>[2x]GEIRPTIGQQMETGDQRFGDLVFRQLAPNVWQHTSYLDMPGFGAVASNGLIVRDGGRVLVVDTAWTDDQTAQILNWIKQEINLPVALAVVTHAHQDKMGGMDALHAAGIATYANALSNQL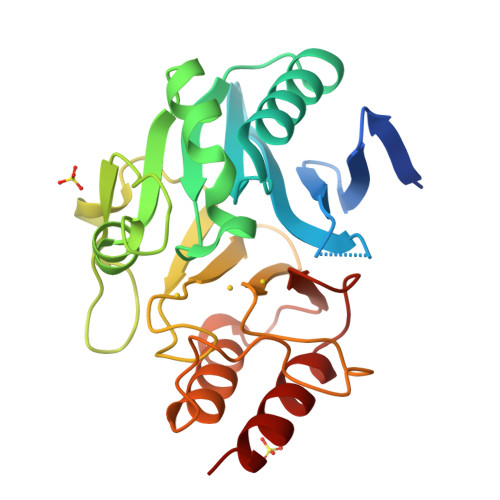APQEGMVAAQHSLTFAANGWVEPATAPNFGPLKVFYPGPGHTSDNITVGIDGTDIAFGGCLIKDSKAKSLGNLGDADTEHYAASARAFGAAFPKASMIVMSHSAPDSRAAITHTARMADKLR>[2x]GLDTVSFSTKGATYITYVNFLNELRVKLKPEGNSHGIPLLRKKCDDPGKCFVLVALSNDNGQLAEIAIDVTSVYVVGYQVRNRSYFFKDAPDAAYEGLFKNTIKTRLHFGGSYPSLEGEKAYRETTDLGIEPLRIGIKKLDENAIDNYKPTEIASSLLVVIQMVSEAARFTFIENQIRNNFQQRIRPANNTISLENKWGKLSFQIRTSGANGMFSEAVELERANGKKYYVT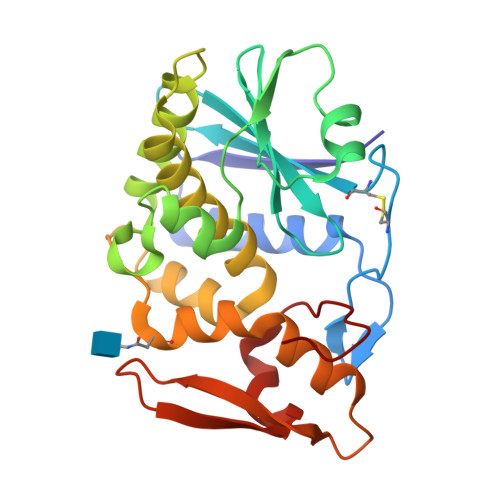AVDQVKPKIALLKFVDKDPK> HMPRVKLGTQGLEVSKLGFGCMGLSGDYNDALPEE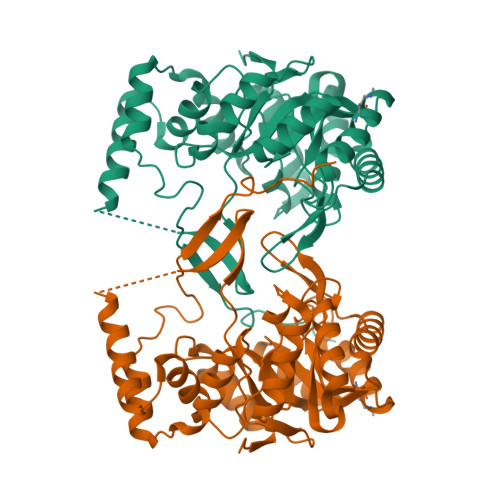QGIAVIKEAFNCGITFFDTSDIYGENGSNEELLGKALKQLPREKIQVGTKFGIHEIGFSGVKAKGTPDYVRSCCEASLKRLDVDYIDLFYIHRIDTTVPIEITMGELKKLVEEGKIKYVGLSEASPDTIRRAHAVHPVTALQIEYSLWTRDIEDEIVPLCRQLGIGIVPYSPIGRGLFAGKAIKESLPENSVLTSHPRFVGENLEKNKQIYYRIEALSQKHGCTPVQLALAWVLHQGEDVVPIPGTTKIKNLHNNVGALKVKLTKEDLKEISDAVPLDEVAGESIHEVIAVTNWKFANTPPL>MSLLEVIIVLGIIGTIAAGVVILAQRAFDSRTVSELVTNTNTIRVAMKDAYQRDGKYPDYQAPLSLTADSIKTDSTGIAVAQLVQLGKLTPDEARNGISGDYIGIGGAITSSGSTINKGFAMELNGLSQEQCRSILGQVGDNWEYVAVGTSPSGSYDALSAGAVNMLAATDN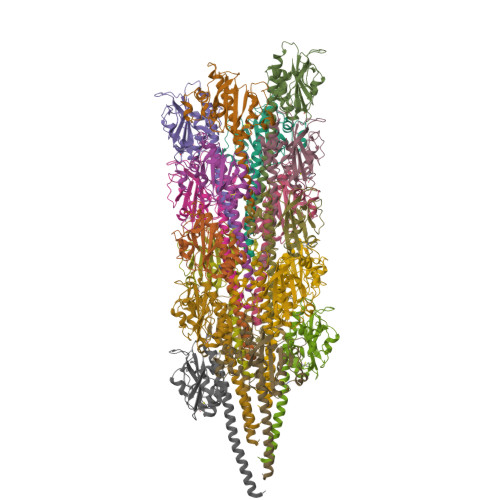TTILRSLAANGQVSLTAEKILKTCTATVNSITLASR[18x]> SPTPLPQLPSNVRDGENNVASTFLQAFFQLWDHDRLTLIPQFYDSETTFSVVFATDSPQDPASSSCSKFSRNLNILSPRHPSTLQRLFVGSNLIADLWKVLPATRHPSLDQTSQWLIDCHTFPHLADPTGMAPYAMGLMINVNGQCEEADISQNLYGTRTFSRCFILGP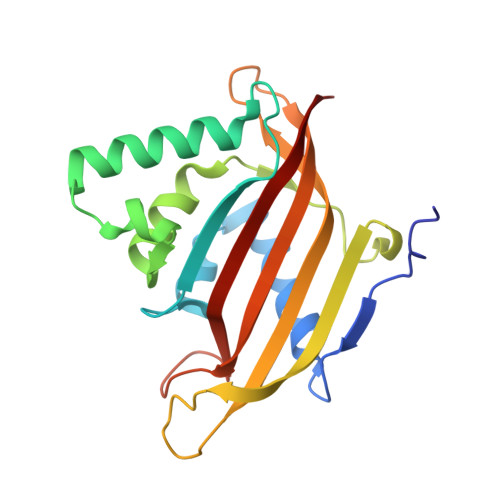SKPGAPHPYRVLSDQLTLHTWKPQ>[18x]MSIQVTGIIEGPLGTPSPGITIRVVSKISYRNTYRLSTEDYVTTTGGAYDFQLNEGFHKILIRYRGASSFTKLGDVSVSDQTPSPITLINLLESSSPKALVVKLQELADEASESAQSASDDADQVTLDKQQVTLLAQQVSDDADQVALDRSATAQSEVNAAQSATTAQQSADDAAAIVPNLQSQIDDKIDKTQSIIPDVDALFSLGRHEINPTNNNIPGLSGTRSLLHIQNNLGGFQLAARTVGSEIHVRSADTNSGNIGPWERLYTTGYRPSSYDLVVKDKAEALSVSHQEGLIIGIESCNGARFVSVLPSDSGGLYLGSLPNGNKLRHIPLDGFSLKTIRTSDFEINSGSDVSQFLIDASTAGYGQVYIDNDCEVTQLCDITGVKYLESLNGAEMLIDDLNGRVKCDTDGFEVKGIVFKKSGDYSNTTFEAYLLETNGEKSLASRCQFVGQWAGYKLQGNDSSADLCFFSDGTFMLRVGEGVSSCNINRCFFTRGTRRFTEGEQQGDGIKLTAQSSTQGYNENIIISDCIFYDTYRDCIDGYVGANRLIVKGSIMLNWGAHALDFKSRVDDNSESPDGGPLTRNVLVDGCMIWKDVVRPDFDLTLAAVVMSVIPGALPVPTSEADVRQNGLRGMELKNTLIAYKGNGSLISAASTWRTVIDGCTLTDLGQIGQIIYAPNSWHLKLINSTVNIDPSNINNVKFSSAMNNAEVNDNTFNRLLISTDGMIRTSIKRNKFNGEGVLSRGLN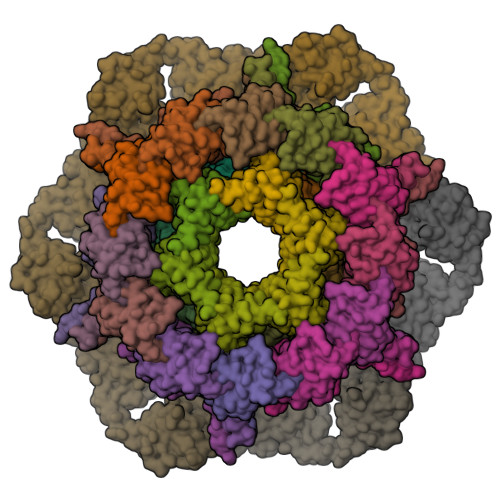IASEEVSAVSNEFENFTSFGAQIFNSASKCRFDFNEIRNCPAPLGIENPSVNTYHSVRGNISMGSGAFTGLNRITDNGGVANGNDHVPYS;>[6x]MLPNMRSALKMFEQSVLLKSVETIRVDFVDDIIITATPIRAVVQVADKKKLNLDSLDWSKQYIWVHSGSKMEIGQFIEWHGKDFKLVAAGDDYSDYGYNAWYGEETLKPVLVSS;>MSQSIINVARYIRDLLDYDENLIQFDRKNTQQSDTVTGYIVVNGSGVQNVLSHGSSYDGDAEIMEYSKSESRLITLEFYGSDAYENAELFSLLNQSQKAKEVSRGLGLTIYNVSQATDVKQLLGYQYGNRVHVDFNIQYCPSVYVETLRVDASEFEILVDD[6x];>[6x]MASISEVIRVSLQQEGRAIAPDNMNAVGIITGNQGVLSTADRYRIYRTAAAVASDFGASSQESAFANTFFDTTPNPISAGGVLVIGYWRSASETVAATSATLVSEQTSESVLIPLLNAINDGSFTITVDGGTEQEVTALDFTGVSELSEVATILNSAITGATVSEDNGYFKVTSSTTGATSLLSYLGVATSGTDISAVLGMNSESGAVLTQGTDQVVLPAETKLEGITAIKSEVNIKGAMFIDQILDADIPGIASFAGANNMLVYEVFDTGYLSKNVSNPVWAVKLAGQSNFRCLLSKSGNRKFAATYMARMHTVLFSGQNTAITMQLKELSVTAEEYTDTEIANAKTVGLDLLTTIKNEQALLTSGANDFCDNVYNLEAFRDEIQTNNYNLLKTTSTKIPQTDPGMDTIEDDTEKTCEKYVRNGVFAPGTWTRSDFFGDRQQFVDAIAQKGYYVLIGDLADQTTAERQSRVSPVIQIAVKNAGAVHEEDIIISVNL;>[6x]MSVIVYRNNQSTLTLNGYTFQHLYQGAALVLTPVNAKTARTNSINGGVSISGRVDGGVHTLAIMVQKHSPDDKFLNDAKNSQEPVVFDGSMKRAYTESGTLKKATTTLETGSITTQPTKTDNNQDPDDSRTYVIEFRNSVETF2-chloro-4-{1'-[(2R)-2-hydroxy-3-methyl-2-(trifluoromethyl)butanoyl]-4,4'-bipiperidin-1-yl}-N,N-dimethylbenzamide | 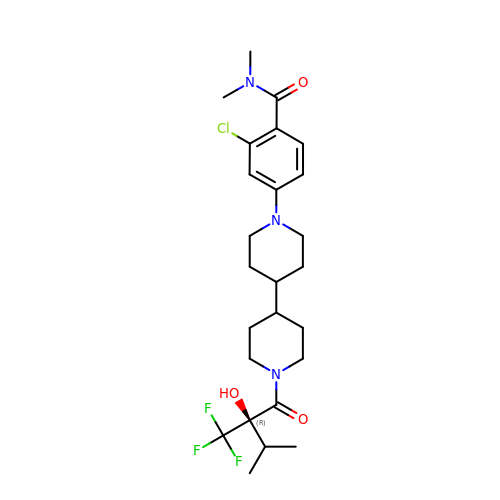C25 H35 Cl F3 N3 O3 | POYRTHYMXFSQBJ-XMMPIXPASA-N(2S)-3-cyclohexyl-2-[4-(methylsulfonyl)-2-oxopiperazin-1-yl]-N-(1,3-thiazol-2-yl)propanamide 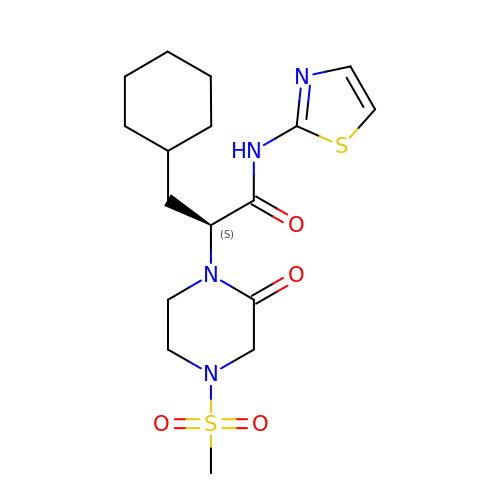| C17 H26 N4 O4 S2 | MCVZXAIMSDHSPP-AWEZNQCLSA-N>AGAGAMNASPQLDHHTELHAAPPLWRPGRVLARLREHQPGPVHIIDPFKVPVTEAVEKAAELTRLGFAAVLLASTDYESFESHMEPYVAAVKAATPLPVVLHFPPRPGAGFPVVRGADALLLPALLGSGDDYFVWKSFLETLAAFPGRIPREEWPELLLTVALTFGEDPRTGDLLGTVPVST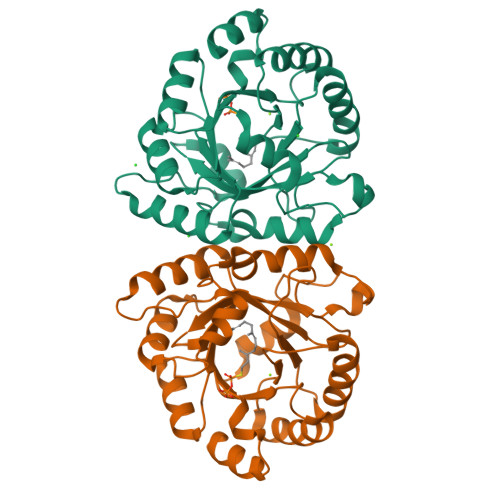ASTEEIDRYLHVARAFGFHMVYLYSRNEHVPPEVVRHFRKGLGPDQVLFVSGNVRSGRQVTEYLDSGADYVGFAGALEQPDWRSALAEIAGRRPAAPARPGSGR[2x]>AETVSFNFNSFSEGNPAINFQGDVTVLSNGNIQLTNLNKVNSVGRVLYAMPVRIWSSATGNVASFLTSFSFEMKDIKDYDPADGIIFFIAPEDTQIPAGSIGGGTLGVSDTKGAGHFVGVEFDTYSNSEYNDPPTDHVGIDVNSVDSVKTVPWNSVSGAVVKVTVIYDSSTKTLSVAVTNDNGDITTIAQVVDLKAKLPERVKFG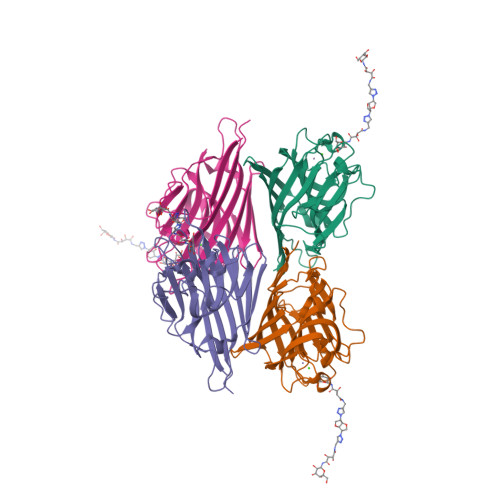FSASGSLGGRQIHLIRSWSFTSTLITTTRRS[4x]> GAD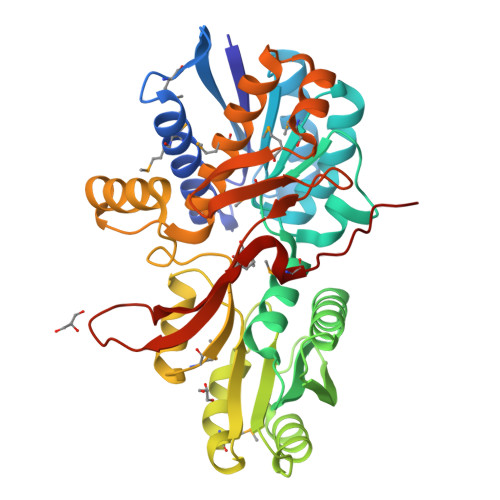DLKIALIYGKTGPLEAYAKQTETGLMMGLEYATKGTMTLDGRKIVVITKDDQSKPDLSKAALAEAYQDDGADIAIGTSSSAAALADLPVAEENKKILIVEPAVADQITGEKWNRYIFRTGRNSSQDAISNAVAIGKQGVTIATLAQDYAFGRDGVAAFKEALAKTGATLATEEYVPTTTTDFTAVGQRLFDALKDKPGKKIIWVIWAGGGDPLTKLQDMDPKRYGIELSTGGNILPALAAYKRLPGMEGATYYYYDIPKNPINEWLVTEHQKRFNAPPDFFTAGGFSAAMAVVTAVQKAKSTDTEKLIAAMEGMEFDTPKGKMVFRKEDHQALQSMYHFKVKVDPAVAWAVLEPVRELKIEEMNIPIKNKK>[2x]MTFTKACSVDEVPPGEALQVSHDAQKV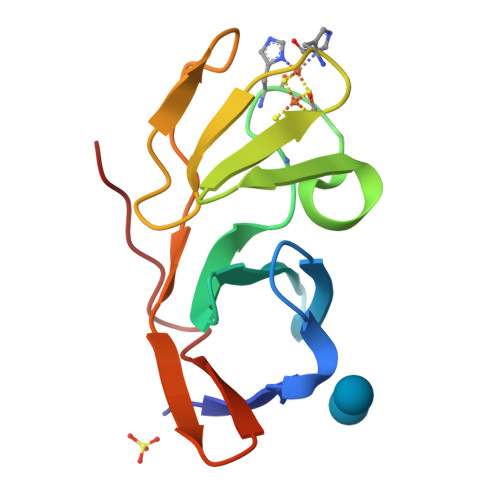AIFNVDGEFFATQDQCTHGEWSLSEGGYLDGDVVECSLHMGKFCVRTGKVKSPPPCEPLKVYPIRIEGRDVLVDFSRAALHA>[2x]GGSLNDLSALTRLPFDRRIEEFFMYLGGRRGTEAVGESREPGVWEVFRYDEAVQVLGDHRTFSSDMNHFIPEEQRQLARAARGNFVGIDPPDHTQLRGLVSQAFSPRVTAALEPRIGRLAEQLLDDIVAERGDKASCDLVGEFAGPLSAIVIA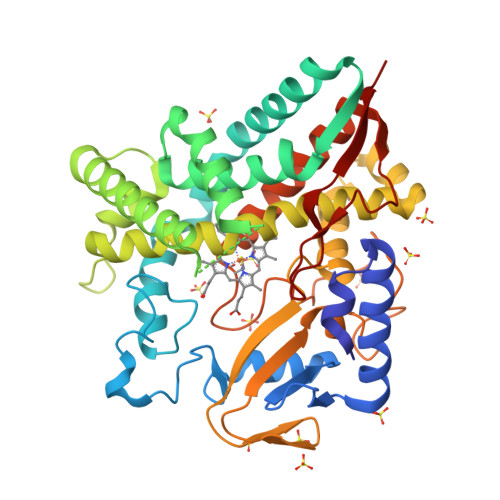ELFGIPESDHTMIAEWAKALLGSRPAGELSIADEAAMQNTADLVRRAGEYLVHHITERRARPQDDLTSRLATTEVDGKRLDDEEIVGVIGMFLIAGYLPASVLTANTVMALDEHPAALAEVRSDPALLPGAIEEVLRWRPPLVRDQRLTTRDADLGGRTVPAGSMVCVWLASAHRDPFRFENPDLFDIHRNAGRHLAFGKGIHYCLGAPLARLEARIAVETLLRRFERIEIPRDESVEFHESIGVLGPVRLPTTLFARR>[2x]SMKHPLEELKDPTENLLL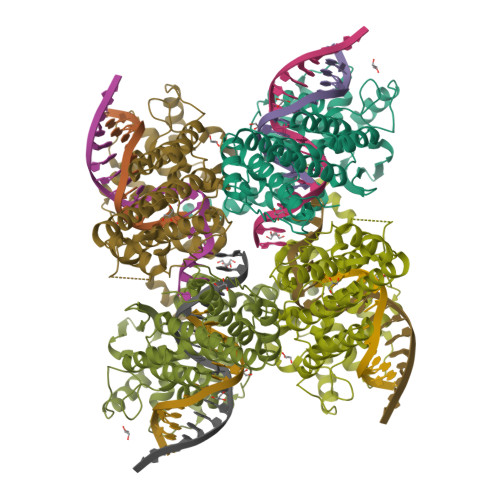WIGRFLRYKCTSLSNSQVKDQNKVFECLNELNQACSSSQLEKVCKKARNAGLLGINTYALPLLKFHEYFSKARLITERLAFNSLKNIDEVMLAEFLSVYTGGLSLATKKNYRIALLGLFSYIDKQNQDENEKSYIYNITLKNISGVNQSAGNKLPTHLNNEELEKFLESIDKIEMSAKVRARNRLLIKIIVFTGMRSNEALQLKIKDFTLENGCYTILIKGKGDKYRAVMLKAFHIESLLKEWLIERELYPVKNDLLFCNQKGSALTQAYLYKQVERIINFAGLRREKNGAHMLRHSFATLLYQKRHDLILVQEALGHASLNTSRIYTHFDKQRLEEAASIWEEN> MATPSMMPQWSYMHISGQDASEYLSPGLVQFARATETYFSLNNKFRNPTVAPTHDVTTDRSQRLTLRFIPVDREDTAYSYKARFTLAVGDNRVLDMASTYFDIRGVLDRGPTFKPYSGTAYNALAPKGAPNPCEWDEAATALEINLEEEDDDNEDEVDEQAEQQKTHVFGQAPYSGINITKEGIQIGVEGQTPKYADKTFQPEPQIGESQWYETEINHAAGRVLKKTTPMKPCYGSYAKPTNENGGQGILVKQQNGKLESQVEMQFFSTTEATAGNGDNLTPKVVLYSEDVDIETPDTHISYMPTIKEGNSRELMGQQSMPNRPNYIAFRDNFIGLMYYNSTGNMGVLAGQASQLNAVVDLQDRNTELSYQLLLDSI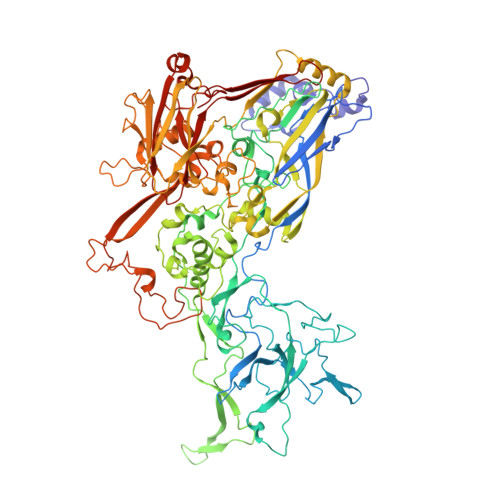GDRTRYFSMWNQAVDSYDPDVRIIENHGTEDELPNYCFPLGGVINTETLTKVKPKTGQENGWEKDATEFSDKNEIRVGNNFAMEINLNANLWRNFLYSNIALYLPDKLKYSPSNVKISDNPNTYDYMNKRVVAPGLVDCYINLGARWSLDYMDNVNPFNHHRNAGLRYRSMLLGNGRYVPFHIQVPQKFFAIKNLLLLPGSYTYEWNFRKDVNMVLQSSLGNDLRVDGASIKFDSICLYATFFPMAHNTASTLEAMLRNDTNDQSFNDYLSAANMLYPIPANATNVPISIPSRNWAAFRGWAFTRLKTKETPSLGSGYDPYYTYSGSIPYLDGTFYLNHTFKKVAITFDSSVSWPGNDRLLTPNEFEIKRSVDGEGYNVAQCNMTKDWFLVQMLANYNIGYQGFYIPESYKDRMYSFFRNFQPMSRQVVDDTKYKDYQQVGILHQHNNSGFVGYLAPTMREGQAYPANFPYPLIGKTAVDSITQKKFLCDRTLWRIPFSSNFMSMGALTDLGQNLLYANSAHALDMTFEVDPMDEPTLLYVLFEVFDVVRVHRPHRGVIETVYLRTPFSAGNATT>[2x]GPQTLVNSLEFLNIQKNSTMS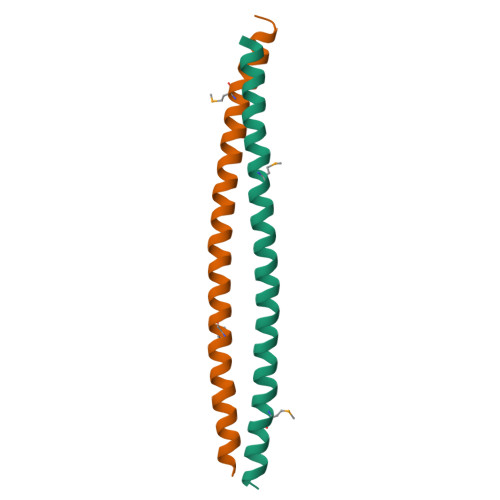EIRDIEVEVENLRQKKEKLLGKIANIEQNQLMLEDNLKQIDDRLDFLEEYG>[2x]MGIEYSNPKDKVEEFEIVNEVEKKSEKRCKEINILSFREAMIRSQILGLIDNYDYEGALNLVSNQKSFRNGKLLRKKLLSLTKQIKTHEVFPEINEKYRDDALKKSLFHYLLLNMRYNRLDVAETLIRVKSIAEFIL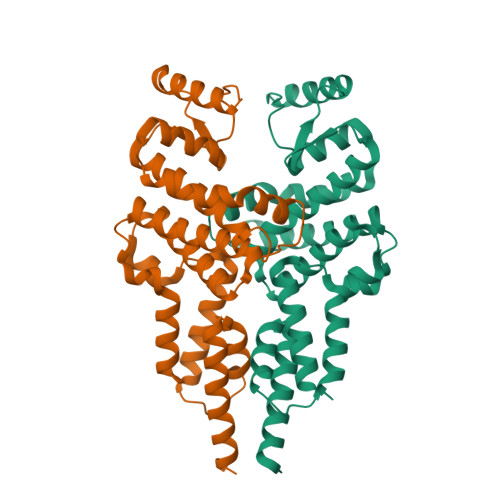KTYIEIHWPTLIIEKDGKPYLNDEDNLSFVYKYNLLLEKRKQNFDVSRILGLPAFIDILTILEPNSQLLKEVNAVNDINGLRNSIAHNLDTLNLDKNKNYKKIMLSVEAIKNMLHISFPEIEEEDYNYFEEKNKEFKELLEHHHHHH>MTKHYDYIAIGGGSGGIASINRAAMYGQKCALIEAKELGGTCVNVGCVPKKVMWHAAQIREAIHMYGPDYGFDTTINKFNWETLIASRTAYIDRIHTSYENVLGKNNVDVIKGFARFVDAKTLEVNGETITADHILIATGGRPSHPDIPGVEYGIDSDGFFALPALPERVAVVGAGYIAVELAGVINGLGAKTHLFVRKHAPLRSFDPMISETLVEVMNAEGPQLHTNAIPKAVVKNTDGSLTLELEDGRSETVDCLIWAIGREPANDNINLEAAGVKTNEKGYIVVDKYQNTNIEGIYAVGDNTGAVELTPVAVAAGRRLSERLFNNKPDEHLDYSNIPTVVFSHPPIGTVGLTEPQAREQYGDDQVKVYKSSFTAMYTAVTTHRQPCRMKLVCVGSEEKIVGIHGIGFGMDEMLQGFAVALKMGATKKDFDNTVAIHPTAAEE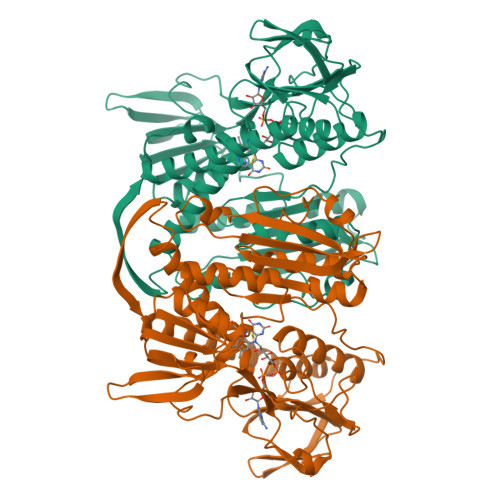FVTMR[2x]>MKRHLILLFVGVSLPFLLAAQQKNSVSITKRVLRIPEVTVVGKRPMKDIGVQRTRFDSIAMKENIALSMADVLTFNSSVFVKNYGRATLSTVAFRGTSPSHT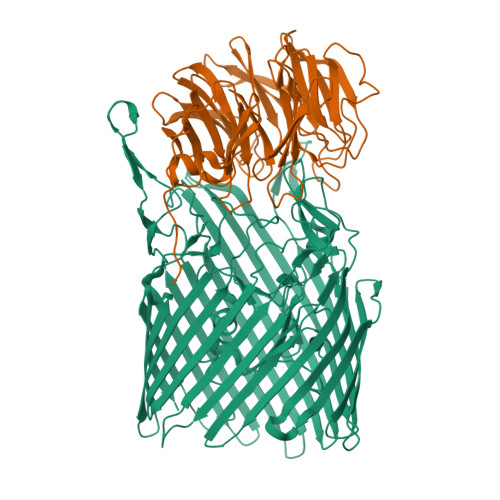QVTWNGMRINNPMLGMTDFSTIPSYFIDDASLLHGTSSVNETGGGLGGLVRLSTSPANHEGFGLQYVQGVGSFSTFDEFLRLTYGDKHWQSSTRVVYSSSPNDYKYRNRDKKENIYDEDKNIIGSYYPTERNRSGAYKDLHVLQEIYYNTGEGDKFGLNAWYINSNRELAMLSTDYGNDMDFENRQREQTFRGVLSWDRVREKWKVGVKGGYIHTWMAYDYKRDKGNGEMASMTRSRSKINTFYGSADGDYAPSEKWLFTAGVSVHQHLVESADKNIISQEGNKAVVGYDKGRVEFSGSVSAKWRPVDRFAASLVLREDMFGTEWAPVIPAFFIDGVLSKKGNIVAKASISRNYRFPTLNDLYFLPGGNPDLKSEHGFTYDVGLSFSVGKENVYALSGGINWFDSHIDDWIIWLPTTKGFFSPRNLKKVHAYGAETNAHLDIMLGKDWKLDMNGTFSWTPSINESEPMSPADQSVGKQLPYVPEFSATVTGRLSWRTWSLLYKWCYYSQRYTMSSNDYTLTGYLPPYFMNNVTLEKQLSFRWADLSLKGSINNLFDEEYLSVLSRPMPGINFEIFIGITPKFGKNKNSKRHHHHHH[3x];>MIRVLFFIRMTMSRTIQRICLFLFCLPVFGSCMKWDYGEMEDFSVSASGLFITNEGNFQYSNATLSYYDPATCEVENEVFYRANGFKLGDVAQSMVIRDGIGWIVVNNSHVIFAIDINTFKEVGRITGFTSPRYIHFLSDEKAYVTQIWDYRIFIINPKTYEITGYIECPDMDMESGSTEQMVQYGKYVYVNCWSYQNRILKIDTETDKVVDELTIGIQPTSLVMDKYNKMWTITDGGYEGSPYGYEAPSLYRIDAETFTVEKQFKFKLGDWPSEVQLNGTRDTLYWINNDIWRMPVEADRVPVRPFLEFRDTKYYGLTVNPNNGEVYVADAIDYQQQGIVYRYSPQGKLIDEFYVGIIPGAFCWK[3x]>[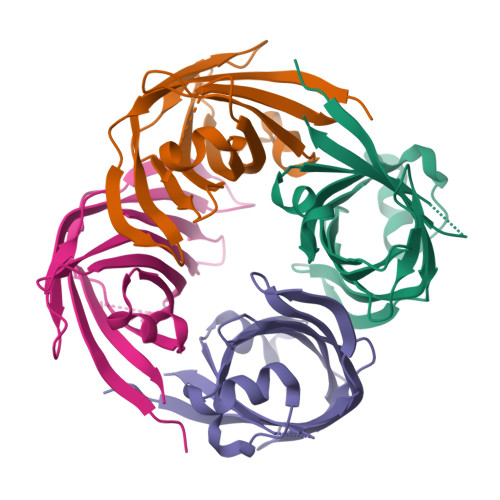8x]MDITNIKEMNYEEVFSITITVDKPILIGQDDIVGRRQLIPIISGKVSGNNFNGKVLPGGIDSQIVRPDGKCELSARYAIRLDDGAAIYIENNGIRTVPDEYIEAVKSGEFVDPNAYYFRTIPTFETYSPKYKWMMNHIFVCCASRLPENVLLKFYKIS>[2x]MNSLLRLPALKRGVFTMSKRGLATTVSPKTRTSNLKNGLTIASESNPLVQTATVGVWIDAGSRNENAYNNGTAHFFEHLAFKGTDKRSQHQLELDIENMGGHLNAYTSRESTVYYAKSFKDDVPKSVEILADILQHSKLAESAIDREREVITRELEEVNKQYEEVVFDHLHATAFMNQPLGRTILGPRENIQTITNTELRKFITENYTADRMVLVGAGAVDHDALVELAEKYFSHLPSSQSPVPLGTPRSSGEDANQNPIPNFVGSEVRLRDDTMPVAHIAIAVEGVSWTSEDYYTALVAQAIIGNYDRAVGTSRHQGSRLSNIVSENNLANSFQSFSTSYSDTGLWGIYLTSENTTQIDDLVHFTLKEWNRLSTSVSNLQVERAKSQLKAGLLLSLDGTTYVAEDIGRQLTTLGRRVTPAEVEAKLEAVTEHDVRAWAQKTLYDKDIALVGLGPIEGLYDYNRIRNDMSMMRW;>MTRGVPRLAVAARHFSTAEAAGVKVAAQDGQSPISDLSVVLRGGSRYATVPGVSHILEKFAFQNTVPKSALRFVRELELFGGKLYTHTTREHIVLRTQFLKQDLPYFVDAFANVLKETKFQQFELTERVAPVAELDLLKRESDPAFTALEAAHEVAFRTGLGNSVYAQGYSPVTLEDVKEFARQVYAKQNVAVVGNNVVPADLQQLVGTAFADLQEGSKVTQAGTTTLHGGEARVRTS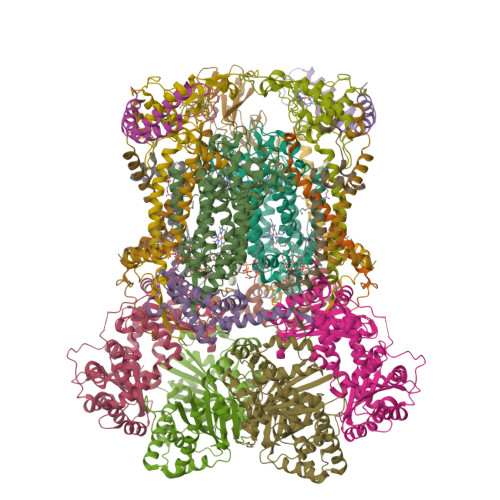TGNALTIALPIAEPKPVYHALASFLGGPASMPWSVGASPLAQATVGTHTSVKATYHNYGDAGLFAITIKGDSPAEISQVAHKAVQALKDTGAEVTEEQAARAYAKSKFAAAEAFENPDSSASVIGMELLSGVSRIAPENVQKFTPAELSEAAAQLSASAKPVVAAVGQVHALPFADELF[2x];>MALRKKNSLLNMANSYVLDSPQPSNLNYFWNFGSLLALCLVIQLATGITLAMHYTSHASLAFDSVEHIMRDVNFGWFIRYAHANTASFFFICIYAHMGRNIYYGSYKTPRVLPWSIGVIIFLLLIITAFMGYVLVFGQMSLWGATVICNLVSAIPWLGEDIVHFLWGGFSVGNPTLQRFFALHYLMPFVLAVFALLHLIALHTAGSSNPLGITSNVDKLSMHPYYSFKDLITVFAFLLMFTLFVFFSPDKLGHPDNYIPANPMVTPASIVPEWYLLPFYAILRAIPDKLGGVIAMVAAILILLILPIVDRSIIRGNAFKPISKLLFGFFICNFLLLGVLGQVHIEPPFIVLGQICTIFYFSYFLILLPMVSTIENIFFYIGSLRK[2x];>MRRRRIGVWPENRRVSRLWVSLSPRSCVTCPVPTNQNPPINNHHTPILTQMFKAIPLRQALLGISSAVCAGATTTYYYTTKAEAMTAAEHGLHPAEYPWPQNGMLSTFDHASLRRGYQVYKEVCAACHSLDRIAWRNLVGVTHTTDEAKAFAEELEYDDEPDDEGNPRKRPGKLADYIPGPYPNEQAARAANQGALPPDLSLIAKARHGGADYIFALLTGYPDEPPAGVVLAPGMNYNPYFPGGGIGMARTLFDGVVEYEDGTPATTSQMAKDVAAFLTWAAEPEHDERKKLGLKAIIVISAMLGLSVYIKKFKWSPIKNRKFIYNPPKN[2x];>[2x]MSLLRTAAQAVKAPKAYTPLVAAKAFAQTRSVSSQPIGGKSTYKIPDFTPYLKKDRNTDANRLFSYFMIGSFGMLSAAGAKATVQDFLSNMSASADVLAMAKVEVKLGAIPLGKNVIIKWRGKPIFIRHRTSEEIEEANEVNVATLRDPQTDDERVQKPEWLVMIGVCTHLGCVPIGEAGDFGGWFCPCHGSHYDISGRIRRGPAPLNLEIPEYDFADAETLVIG;>[2x]MSYFLTLASEVAESLLPTVAFASEEEKEQDEPVEVESDDDESEEKEDDDEEEDEDDDDDDDDDEVPDPAIALHEAAAEGPCHDFKHHFDECVERVTKAQEAEDYDHAEYKEDCVEEFFHLQHCINDNTADKLFRVLK;>[2x]MASITSVVKTSELILKSPLLSKIVVPLAKTYVKFSGYRQLGFKMNDLIIEETPNMQLALRRLPPTESYDRVYRLIRATQFSLSHKLATGNDITKPEEDDHYLIPYILDVEAEAFEKDALDNLEVVKRK;>MGGNGHYMGWWGHMGSPPQKGIAGYTISPFAARPFAGVVHAAIFNTFRRTKNQALFVILPVSFFYYVWTQASEKNEWLYTKAGRHELAKALAE[2x];>MAWATTFYNVFVKRNSAFVATILASAFVFDMTFETAIDNFWDRINAGKQWKDIRHKYIEAAGDDDEDDE[2x];>[2x]MICGEGDYVKKPSYKIVPHFLGFNIPTVSKWIPIFGIWGAAAGIGALFLIEGVPRTRQDILSKIPIIGEHWIREIPASDNPF> MAFVSGAGAAVRGTSGKAAARCAAVRTVRAARAIRMTTAPGSAPFSSLDEPERQVVMWESVGDEKDQVFKQLYRQVFGNAYLMESDLEELLVPESQLLMGSISVKDFIKRVAKSDAYKKRFFEPCGPYRFVELCTKHFLGRGPRDQKEVSEHVQRLANEGYDADVDSYMDSEEYMSLFGENGVPRFVFKGTYEGNDQFNRLAAMRQFADGSYTDTRSGSTAPRKAQKAELTMAEGDFVGRAKVSRGLPAETSAAKTGTPPVRALKGPVNPRAGVRVRIKVVDNLYQVYEIPPMADPKAKVNAFWAKPIPSSLTKKY;> MLDAFSRVVVNSDAKAAYVGGSDLQALKSFIADGNKRLDAVNSIVSNASCMVSDAVSGMICENPGLISPGGNCYTNRRMAACLRDGEIILRYVSYALLAGDASVLEDRCLNGLKETYIALGVPTNSSIRAVSIMKAQAVAFITNTATERKMSFAAGDCTSLASEVASYFDRVGAAIS

Red algae utilise a megadalton-size light harvesting antenna called the red algal phycobilisome (PBS)—comprised of rod structures formed from stacked, hexameric protein-pigment rings emanating from a protein core that is poised above an integral membrane photosystem. Published cryo-EM maps for two red algal phycobilisomes contain clusters of unmodelled density homologous to the cryptophyte-αβ protomer. We modelled these densities, identifying a new family of scaffolding proteins related to red algal phycobilisome linker proteins that possess multiple copies of a cryptophyte-α-like domain. These domains bind to, and stabilise, a conserved hydrophobic surface on phycoerythrin β, which is the same binding site for its primary partner in the red algal phycobilisome, phycoerythrin α.

16 of these apparently ‘lone’ PE β subunits (with no PE α partners) are conserved between the two red algal PBS structures (which equates to 8 pairs of PE β subunits in each as both red algal PBS has two-fold symmetry). Of these conserved ‘lone’ PE β subunits, three pairs are bound to other red algal PBS proteins. The 6 non-CALM bound ‘lone’ PE β subunits also appear to have found ways to cope with this patch, either through truncation or by co-opting alternative binding partners. This includes a new linker protein, Linker 3, which we have modelled. LR2, “Linker 3”, LR3 and LR6 retain C-terminal domains with some similarity to Pfam01383.>MAKSYKSVALVVGVTGIVGSSLAEVLKLPDTPGGPWKVYGVARRPCPVWLAKKPVEYIQCDVSDNQETISKLSPLKDITHIFYVSWIGSEDCQTNATMFKNILNSVIPNASNLQHVCLQTGIKHYFGIFEEGSKVVPHDSPFTEDLPRLNVPNFYHDLEDILYEETGKNNLTWSVHRPALVFGFSPCSMMNIVSTLCVYATICKHENKALVYPGSKNSWNCYADA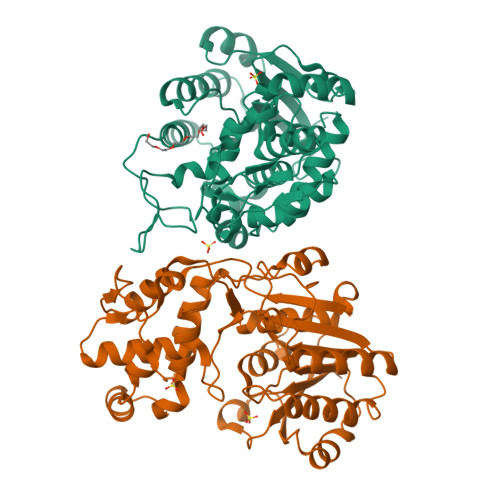VDADLVAEHEIWAAVDPKAKNQVLNCNNGDVFKWKHIWKKLAEEFGIEMVGYVEGKEQVSLAELMKDKDQVWDEIVKKNNLVPTKLKEIAAFWFADIAFCSENLISSMNKSKELGFLGFRNSMKSFVSCIDKMRDYRFIP[2x]>[2x]NSFVGLRVVAKWSSNGYFYSGKITRDVGAGKYKLLFDDGYECDVLGKDILLCDPIPLDTEVTALSEDEYFSAGVVKGHRKESGELYY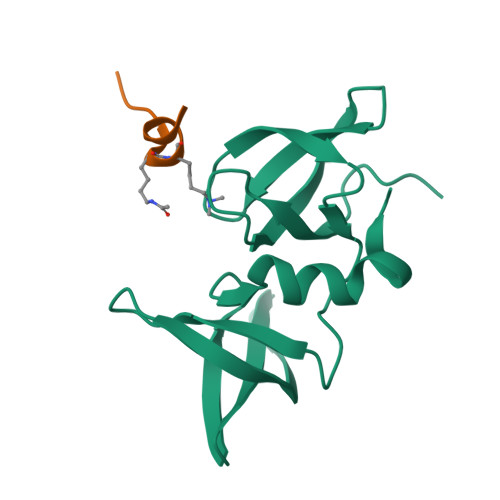SIEKEGQRKWYKRMAVILSLEQGNRLREQYGLG;>TSRHKKLMFK[2x]> MPELTRRHALGAAAALAAVAGTQALAAPSASAAGHHGGPQPFDEVYQGRRIEGRATGGGHHHGSGYGVFIDGMELHVMQNVDGSWISVVSHYDPVATPRAAARAAVVELQGAPLVPFN;> MGSHHHHHHSERTVRKNQATLTADEKRRFVDALVALKRSGRYDEFVTTHNAFIMGDTDSGERTGHRSPSFLPWHRRFLIEFEQALQAVDPSVALPYWDWSTDRTARASLWAPDFLGGSGRSLDGRVMDGPFAASTGNWPVNVRVDSRTYLRRT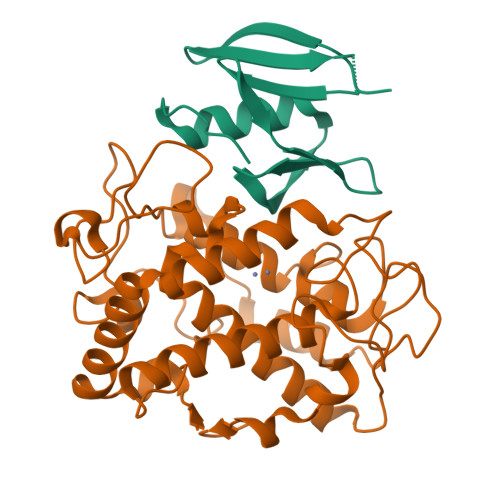LGGGGRELPTRAEVDSVLAMSTYDMAPWNSASDGFRNHLEGWRGVNLHNRVHVWVGGQMATGVSPNDPVFWLHHAYIDRLWAQWQSRHPGSGYVPTGGTPNVVDLNETMKPWNDVRPADLLDHTAHYTFDTV>GASRGLEPSADAPEPDCGDPPPVAPSRLLPLKPVQAATPSRTDPLVLVFVESLYSQLGQEVVAILESSRFKYRTEIAPGKGDMPTLTDKGRGRFALIIYENILKYVNLDAWNRELLDKYCVAYGVGIIGFFKANENSLLSAQLKGFPLFLHSNLGLKDCSINPKSPLLYVTRPSEVEKGVLPGEDWTVFQSNHSTYEPVLLAKTRSSESIPHLGADAGLHAALHATVVQDLGLHDGIQRVLFGNNLNFWLHKLVFVDAVAFLTGKRLSLPLDRYILVDIDDIFVGKEGTRMKVEDVKALFDTQNELRAHIPNFTFNLGYSGKFFHTGTNAEDAGDDLLLSYVKEFWWFPHMWSHMQPHLFHNQSVLAEQMALNKKFAVEHGIPTDMGYAVAPHHSGVYPVHVQLYEAWKQVWSIRVTSTEEYPHLKPARYRRGFIHNGIMVLPRQTCGLFTHTIFYNEYPGGSSELDKIINGGELFLTVLLNPISIFMTHLSNYGNDRLGLYTFKHLVRFLHSWTNLRLQTLPPVQLAQKYFQIFSEEKDPLWQDPCEDKRHKDIWSKEKTCDRFPKLLIIGPQKTGTTALYLFLGMHPDLSSNYPSSETFEEIQFFNGHNYHKGIDWYMEFFPIPSNTTSDFYFEKSANYFDSEVAPRRAAALLPKAKVLTILINPADRAYSWYQHQRAHDDPVALKYTFHEVITAGSDASSKLRALQNRCLVPGWYATHIERWLSAYHANQILVLDGKLLRTEPAKVMDMVQKFLGVTNTIDYHKTLAFDPKKGFWCQLLEGGKTKCLGKSKGRKYPEMDLDSRAFLKDYYRDHNIELSKLLYKMGQTLPTWLREDLQNTRNNNNNNGHHHHHHHH[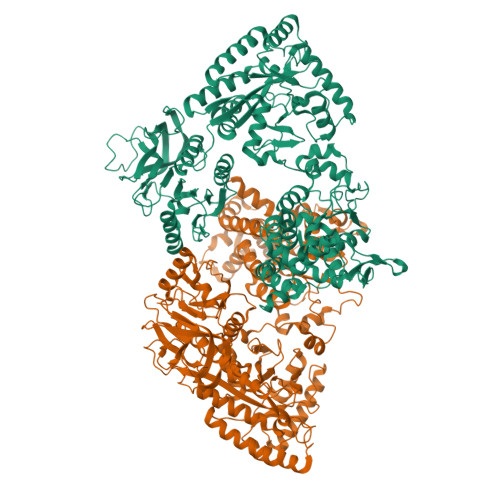2x]> MSDKIIHLTDDSFDTDVLKADGAILVDFWAEWCGPCKMIAPILDEIADEYQGKLTVAKLNIDQNPGTAPKYGIRGIPTLLLFKNGEVAATKVGALSKGQLKEFLDANLAAALVQQLPKAIIIGVRKGGTRALLEMLNLHPAVVKASQEIHFFDNDENYGKGIEWYRKKMPFSYPQQITIEKSPAYFITEEVPE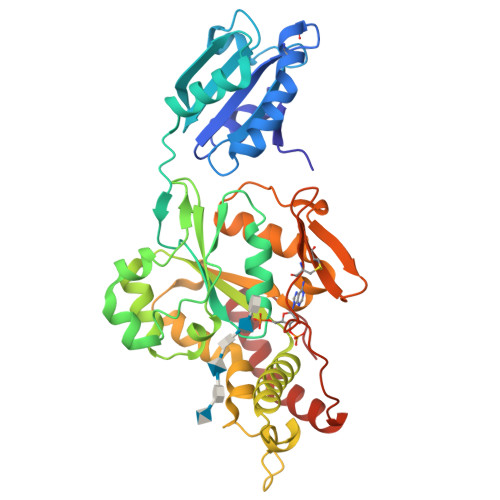RIYKMNSSIKLLIIVREPTTRAISDYTQVLEGKERKNKTYYKFEKLAIDPNTCEVNTKYKAVRTSIYTKHLERWLKYFPIEQFHVVDGDRLITEPLPELQLVEKFLNLPPRISQYNLYFNATRGFYCLRFNEIFNKCLAGSKGRIHPEVDPSVITKLRKFFHPFNQKFYQITGRTLNWP>[10x]MHTKGPTPQQHDGSALRIGIVHARWNETIIEPLLAGTKAKLLACGVKESNIVVQSVPGSWELPIAVQRLYSASQLQTPSSGPSLSAGDLLGSSTTDLTALPTTTASSTGP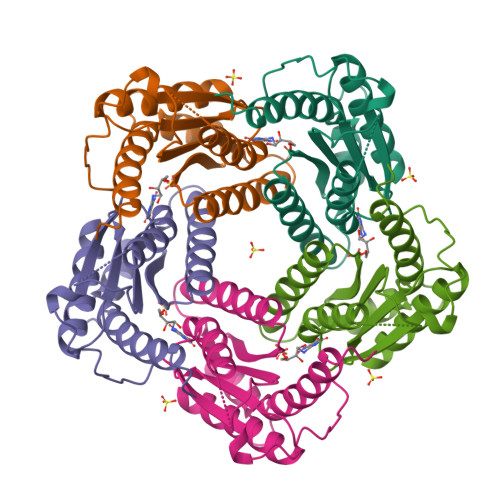FDALIAIGVLIKGETMHFEYIADSVSHGLMRVQLDTGVPVIFGVLTVLTDDQAKARAGVIEGSHNHGEDWGLAAVEMGVRRRDWAAGKTE>NDIKSKDATFASGTLDLSAKENSASVNLSNLKPGDKLTKDFQFENNGSLAIKEVLMALNYGDFKANGGSNTSPEDFLSQFEVTLLTVGKEGGNGYPKNIILDDANLKDL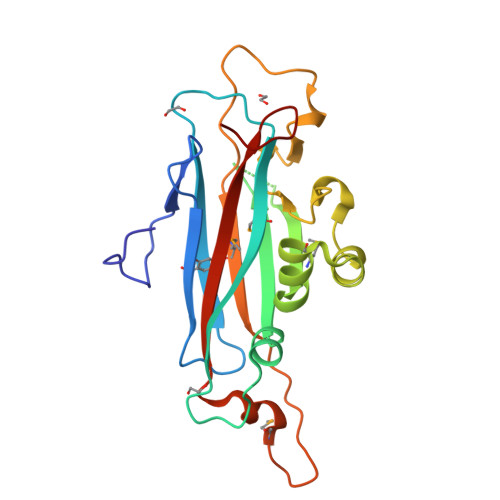YLMSAKNDAAAAEKIKKQIDPKFLNASGKVNVATIDGKTAPEYDGVPKTPTDFDQVQMEIQFKDDKTKDEKGLMVQNKYQGNSIKLQFSFEATQWNGLTIK[2x]4-{6-[(3R)-3-(3-fluorophenyl)morpholin-4-yl]imidazo[1,2-b]pyridazin-3-yl}benzonitrile 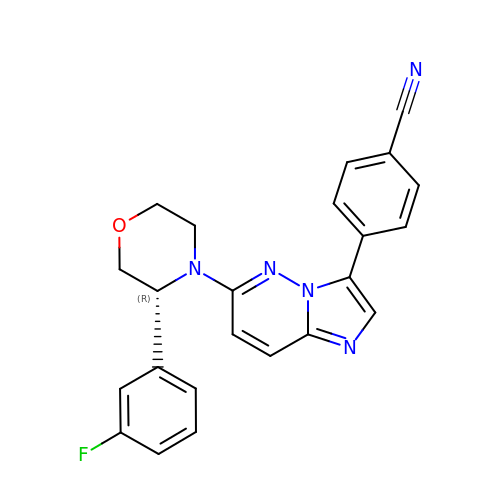| C23 H18 F N5 O | OGLFUDJJJDTBFS-NRFANRHFSA-N>MEEECRVLSIQSHVVRGYVGNRAATFPLQVLGFEVDAVNSVQFSNHTGYSHWKGQVLNSDELQELYDGLKLNHVNQYDYVLTGYTRDKSFLAMVVDIVQELKQQNPRLVYVCDPVMGDQRNGEGAMYVPDDLLPVYREKVV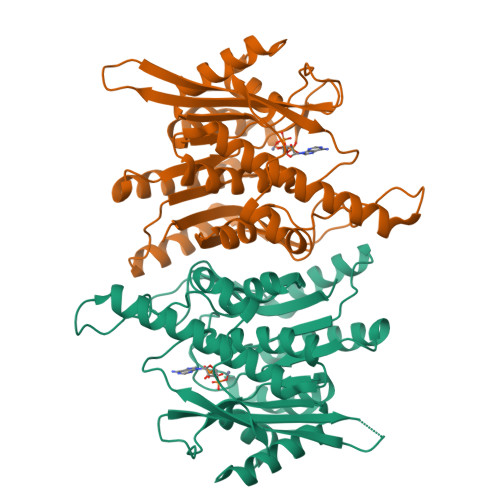PVADIITPNQFEAELLTGRKIHSQEEALEVMDMLHSMGPDTVVITSSNLLSPRGSDYLMALGSQRTRAPDGSVVTQRIRMEMHKVDAVFVGTGDLFAAMLLAWTHKHPNNLKVACEKTVSAMHHVLQRTIKCAKAKSGEGVKPSPAQLELRMVQSKKDIESPEIVVQATVL[2x]> GAVQNDEVAAFCQSIMKLKTKFPYTDHCTNPGYLLSPVTVQRNMCGENASVKVSIEIEGLQLPVTFTCDVSSTVEIIIMQALCWVHDDLNQVDVGSYILKVCGQEEVLQNNHCLGSHEHIQNCRKWDTEIKLQLLTLSAMCQNLARTAEDDEAPVDLNGSGSVMTRHPVEELLD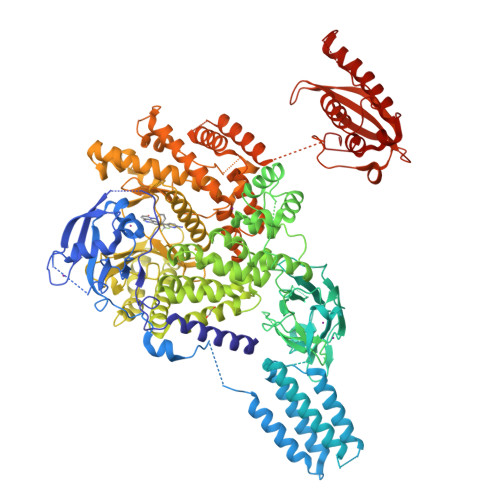SYHYQVELALQTENQHRAVDQVIKAVRKICSALDGVETPSVTEAVKKLKRAVNLPRNKSADVTSLSGSDTRKNSTKGSLNPENPVQVSMDHLTTAIYDLLRLHANSSRCSTGCPRGSRNIKEAWTATEQLQFTVYAAHGISSNWVSNYEKYYLICSLSHNGKDLFKPIQSKKVGTYKNFFYLIKWDELIIFPIQISQLPLESVLHLTLFGVLNQSSGSSPDSNKQRKGPEALGKVSLTLFDFKRFLTCGTKLLYLWTSSHTNSIPGAIPKKSYVMERIVLQVDFPSPAFDIIYTSPQIDRNIIQQDKLETLESDIKGKLLDIIHRDSSFGLSKEDKVFLWENRYYCLKHPNCLPKILASAPNWKWANLAKTYSLLHQWPPLCPLAALELLDAKFADQEVRSLAVSWMEAISDDELADLLPQFVQALKYEIYLNSSLVRFLLSRALGNIQIAHSLYWLLKDALHDTHFGSRYEHVLGALLSVGGKGLREELSKQMKLVQLLGGVAEKVRQASGSTRQVVLQKSMERVQSFFLRNKCRLPLKPSLVAKELNIKSCSFFSSNAMPLKVTMVNADPLGEEINVMFKVGEDLRQDMLALQMIKIMDKIWLKEGLDLRMVIFRCLSTGRDRGMVELVPASDTLRKIQVEYGVTGSFKDKPLAEWLRKYNPSEEEYEKASENFIYSCAGCCVATYVLGICDRHNDNIMLRSTGHMFHIDFGKFLGHAQMFGSFKRDRAPFVLTSDMAYVINGGEKPTIRFQLFVDLCCQAYNLIRKQTNLFLNLLSLMIPSGLPELTSIQDLKYVRDALQPQTTDAEATIFFTRLIESSLGSIATKFNFFIHNLAQLRFSGLPSNDEPILSFSPKTYSFRQDGRIKEVSVFTYHKKYNPDKHYIYVVRILREGHLEPSFVFRTFDEFQELHNKLSIIFPLWKLPGFPNRMVLGRTHIKDVAAKRKIELNSYLQSLMNASTDVAECDLVCTFFHPLLRDEK METTL16 is the second m6A methyltransferase identified, and its known substrates include U6 snRNA and the human MAT2A mRNA that encodes for S-adenosylmethionine (SAM) synthetase (Pendleton et al., 2017). Here we describe the crystal structure of human METTL16 to reveal a methyltransferase domain furnished with an extra N-terminal module, which together form a deep-cut groove that is essential for RNA binding. Consistent with the SAM-dependent methyltransferase activity of METTL16, both structures reveal a Rossmann fold composed of a central seven-stranded β sheet (strands β3–β9) flanked by three α helices each (helices α4–α6 and α7–α9). In contrast, we show here that METTL16 is active as a monomer, and it contains a large deep-cut groove that can accommodate structured RNAs.

Two constructs (core, 1–291 aa; and ΔN, 40–291 aa) encompassing the methyltransferase domain (MTase) were expressed in E. coli and crystallized (Star Methods). First, and most striking, is the presence of an N-terminal module (1–78 aa) in the core structure that is appended to the α4 of the Rossmann fold and that consists of three helices (α1–α3) and two short β strands (β1 and β2). Indeed, when mapped onto the METTL16-core structure, these reveal a positively charged cluster (K5, R10, R12, K14, K16, and R41) that forms the entrance of a wide deep-cut groove. Taken together, our two structures reveal an architecture where the MTase domain is attached to a METTL16-specific N-terminal module that is essential for activity.

>MALSKSMHARNRYKDKPPDFAYLASKYPDFKQHVQINLNGRVSLNFKDPEAVRALTCTLLREDFGLSIDIPLERLIPTVPLRLNYIHWVEDLIGHQDSDKSTLRRGIDIGTGASCIYPLLGATLNGWYFLATEVDDMCFNYAKKNVEQNNLSDLIKVVKVPQKTLLMDALKEESEIIYDFCMCNPPFFANQLEAKGVNSRNPRRPPPSSVNTGGITEIMAEGGELEFVKRIIHDSLQLKKRLRWYSCMLGKKCSLAPLKEELRIQGVPKVTYTEFCQGRTMRWALAWSFYD[2x]> MEDMILTEEMQKIMNLIQDDENNVFVTGKAGSGKTTFLKYLIEKSGKNCIVAAPTGIAAINAGGVTLHSLFGIPFGPITPYDRLENKFSEYKVELLLKMELLIIDEISMVRPDILDTIDRKLRWVYESDEPFGGVQVVMFGDLFQLPPVTKKQEREILSDFYDGFFFFNALVFKRTGFHIVELTKIFRQTEPEFINVL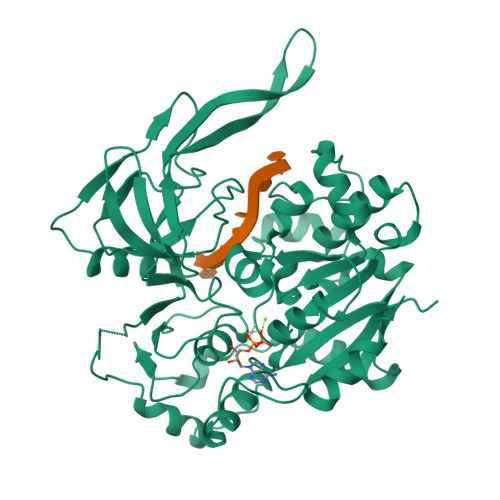NNIRNYQVTSDELDLLSELKDRKISSSYDNEYIHICTHKADVEKINADKLGEQEIRNYDIVIKDKFPESSIPCDLHLKLRVGARVMSLVNDSLKGYYNGMLGIVTALEDNVITVRMDNGRTIKFERYTWSNTQYTLKDNEIVKEEIGSCTQFPLTLAWAITIHKSQGLTFDKIIIHVSHTFCPGQLYVALSRCRTLEGIVSDAFITKQMIIPEYALIDFERAYKSEGNYYGKRLD> MSELEKAVVALIDVFH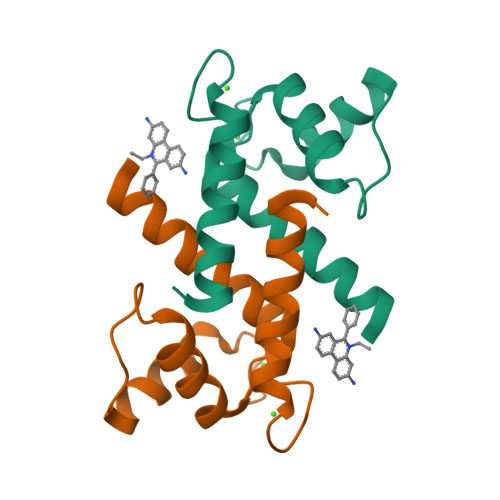QYSGREGDKHKLKKSELKELINNELSHFLEEIKEQEVVDKVMETLDSDGDGECDFQEFMAFVAMITTACHEFFEHE> GSHMEKTGLHVHEKIKHMVKNYGTMITGIPAEILGQNEAEISVGYVKKMGNMKENIAEVVRKSEMTQPTNSAGKASNEVCDLLLGTEGASEFEKSSYQVLSGDGSNLKGSLPNKNLLVRVEMDRFNAPQKYQKIKREEFNPETAEKNKIYLLEDQLVYLDIFGKVIDLGQTSDTCHRLFNAITTPFYQNYILYDEYIDPEESAEEAAMFEMGEIVKAKMKNIDCWTATHSFTIFVPESDSEDTRTLYPYQAYWTSHTLQQWFSGDKDEKLSRLGIDGYIEKLALLGTTTDSKIRSSIYGELFSPPGKEHVFCTGMNEKFSPLRVKFKVTEVNPEIALQNLEEVQEFIDTNYPGENAKDQCELYKIKAQEAMTKQLEMRLLIE;> GSHMFFKDYQKKNVMRLLQDSLEKIINEWLKT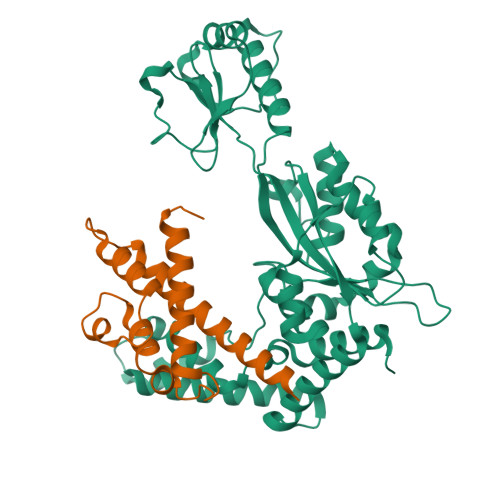DDESHTKLKSLQELSEMDINATSFAEHSPLPDFVTRLWLDPHKALDAMDKNISKNEIRKLIKETAREIELVFTHQK> APPKSVIRWCTISSPEEKKCNNLRDLTQQERISLTCVQKATYLDCIKAIANNEADAISLDGGQAFEAGLAPYKLKPIAAEVYEHTEGSTTSYYAVAVVKKGTEFTVNDLQGKTSCHTGLGRSAGWNIPIGTLLHRGAIEWEGIESGSVEQAVAKFFSASCVPGATIEQKLCRQCKGDPKTKCARNAPYSGYSGAFHCLKDGKGDVAFVKHTTVNENAPDQKDEYELLCLDGSRQPVDNYKTCNWARVAAHAVVARDDNKVEDIWSFLSKAQSDFGVDTKSDFHLFGPPGKKDPVLKDLLFKDSAIMLKRVPSLMDSQLYLGFEYYSAIQSMRKDQLTPSPRENRIQWCAVGKDEKSKCDRWSVVSNGDVECTVVDETKDCIIKIMKGEADAVALDGGLVYTAGVCGLVPVMAERYDDESQCSKTDERPASYFAVAVARKDSNVNWNNLKGKKSCHTAVGRTAGWVIPMGLIHNRTGTCNFDEYFSEG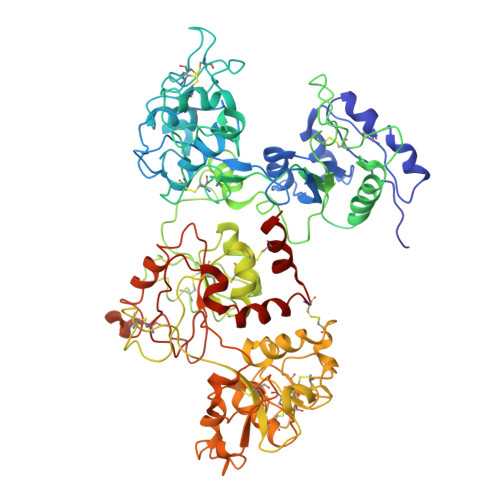CAPGSPPNSRLCQLCQGSGGIPPEKCVASSHEKYFGYTGALRCLVEKGDVAFIQHSTVEENTGGKNKADWAKNLQMDDFELLCTDGRRANVMDYRECNLAEVPTHAVVVRPEKANKIRDLLERQEKRFGVNGSEKSKFMMFESQNKDLLFKDLTKCLFKVREGTTYKEFLGDKFYTVISSLKTCNPSDILQMCSFLEGK> MLQ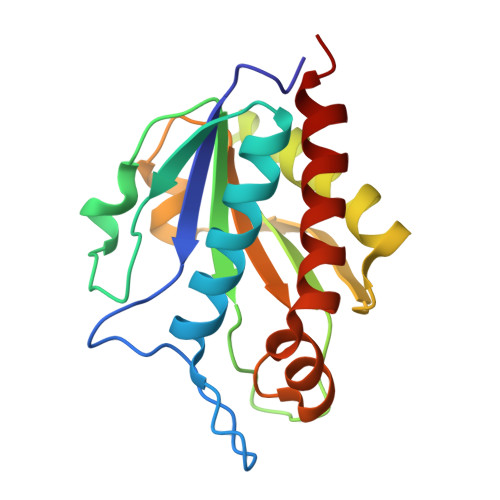GKTIVLDPGHGGSDQGASSNTKYKSLEKDYTLKTAKELQRTLEKEGATVKMTRTDDTYVSLENRDIKGDAYLSIHNDALESSNANGMTVYWYHDNQRALADTLDATIQKKGLLSNRGSRQENYQVLAQTKVPAVLLELGYISNPTDETMIKDQLHRQILEQAIVDGLKIYFSA>MASQQQTVRGWSGINTFAPATQTKLLELLGNLKQEDVN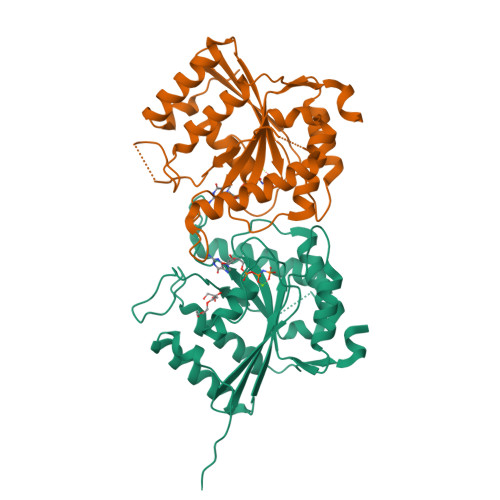SLTILVMGKGGVGKSSTVNSIIGERVVSISPFQSEGPRPVMVSRSRAGFTLNIIDTPGLIEGGYINDMALNIIKSFLLDKTIDVLLYVDRLDAYRVDNLDKLVAKAITDSFGKGIWNKAIVALTHAQFSPPDGLPYDEFFSKRSEALLQVVRSGASLKKDAQASDIPVVLIENSGRCNKNDSDEKVLPNGIAWIPHLVQTITEVALNKSESIFVDKNLIDGPNPNQRGLEHHHHHH[8x]>MSLVVFPFKHEHPEVLLHNVRVAAAHPRVHEVLCIGYERDQTYEAVERAAPEISRATGTPVSVRLQERLGTLRPGKGDGMNTALRYFLEETQWERIHFYDADITSFGPDWITKAEEAADFGYGLVRHYFPRASTDAMITWMITRTGFALLWPHTELSWIEQPLGGELLMRREVAAMLYEDERVRRRSDWGIDTLYTFVTVAAGVSIYECYIPEGKAHRLYGGLDDLRTMLVECFAAIQ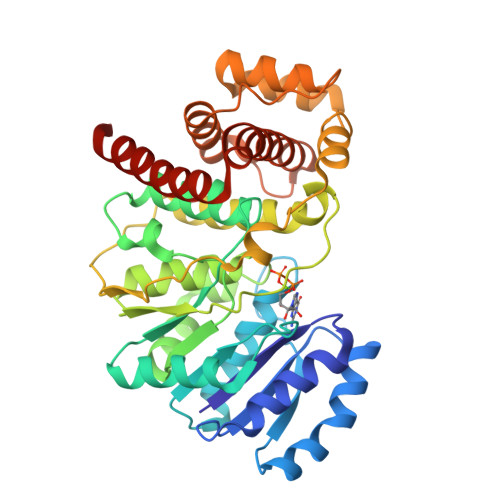SLQHEVVGQPAIHRQEHPHRVPVHIAERVGYDVEATLHRLMQHWTPRQVELLELFTTPVREGLRTCQRRPAFNFMDEMAWAATYHVLLEHFQPGDPDWEELLFKLWTTRVLNYTMTVALRGYDYAQQYLYRMLGRYRYQAALEN[2x]>MMSKIFDLVVIGAGSGGLEAAWNAATLYKKRVAVIDVQMVHGPPFFSALGGTCVNVGCVPKKLMVTGAQYMEHLRESAGFGWEFDRTTLRAEWKNLIAVKDEAVLNINKSYDEMFRDTEGLEFFLGWGSLESKNVVNVRESADPASAVKERLETEHILLASGSWPHMPNIPGIEHCISSNEAFYLPEPPRRVLTVGGGFISVEFAGIFNAYKPKDGQVTLCYRGEMILRGFDHTLREELTKQLTANGIQILTKENPAKVELNADGSKSVTFESGKKMDFDLVMMAIGRSPRTKDLQLQNAGVMIKNGGVQVDEYSRTNVSNIYAIGDVTNRVMLTPVAINEAAALVDTVFGTTPRKTDHTRVASAVFSIPPIGTCG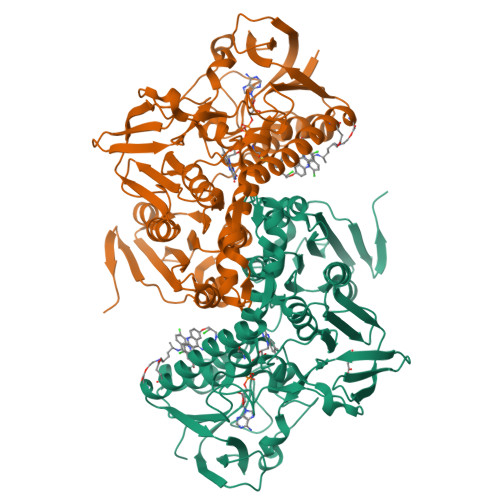LIEEVASKRYEVVAVYLSSFTPLMHKVSGSKYKTFVAKIITNHSDGTVLGVHLLGDNAPEIIQGIGICLKLNAKISDFYNTIGVHPTSAEELCSMRTPSYYYVKGEKMEKPSEASL[2x]>MQEEPTNIPRPDNAELLVASEVAIENAAIALSEIVSVVNTSDGRIEVFGVGTDNAVWHNRQTAPHSGSSWTGWISLNGKVTSKPVVYINTDGRLEVFARGTDNALWHIWQTATNAGWSNWQSLGGTITSNPAVYVNTDGRIDVFARGTDNALWHISQTAAHSGPWSSWQSLNGVITSNPAVHINSDGRLEVFARGTDNALWHIWQTAPDSNQWSGWDSLGGVITSDPVVIGTADGRLEVFARGSNNALYHIWQTVPHGGPWSNWASLNGVITSAPAVVKNSDGRLEVFARGTNNALYHIWQTVSHSGPWSNWATL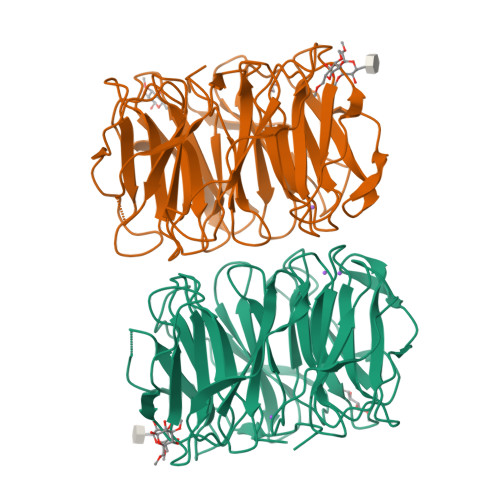NGTITSAPTAVEDADGRLEVFARGTDNALWNIWQATPSWSAWVSLKGSLIDASAIK[2x]>MDVNQQYNHFLKQHVDGEMTTLKCKSQMEILNLNRPDRKCKLKNTFILANPDQVQAICTGGGTLKGNNLVQSNKPFSVVICTHTGGESHPNCTYK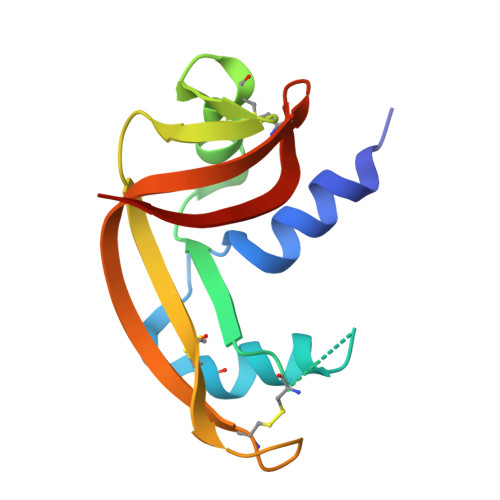GSSATKKVIIACDGKFPVHYDGITDGK[4x]> EPAENSDFYLPGDYLLGGLFSLHANMKGIVHLNFLQVPMCKEYEVKVIGYNLMQAMRFAVEEINNDSSLLPGVLLGYEIVDVCYISNNVQPVLYFLAHEDNLLPIQEDYSNYSSRVVAVIGPDNSESVMTVANFLSLFLLPQITYSAISDELRDKVRFPALLRTTPSADHHIEAMVQLMLHFRWNWIIVLVSNDTYGRDNGQLLGERVARRDICIAFQETLPTLQPNQNMTSEERQRLVTIVDKLQQSTARVVVVFSPDLTLYHFFNEVLRQNFTGAVWIASESWAIDPVLHNLTELRHLGTFLGITIQSVPIPGFSEFREWGPQAGPPPLSRTSQSYTCNQECDNCLNATLSFNTILRLSGERVVYSVYSAVYAVAHALHSLLGCDKSTCTKRVVYPWQLLEEIWKVNFTLLDHQIFFDPQGDVALHLEIVQWQWDRSQNPFQSVASYYPLQRQLKNIQDISWHTINNTIPMSMCSKRCQSGQKKKPVGIHVCCFECIDCLPGTFLNHTEDEYECQACPNNEWSYQSETSCFKRQLVFLEWHEAPTIAVALLAALGFLSTLAILVIFWRHFQTPIVRSAGGPMCFLMLTLLLVAYMVVPVYVGPPKVSTCLCRQALFPLCFTICISCIAVRSFQIVCAFKMASRFPRAYSYWVRYQGPYVSMAFITVLKMVIVVIGMLATGLSPTTRTDPDDPKITIVSCNPNYRNSLLFNTSLDLLLSVVGFSFAYMGKELPTNYNEAKFITLSMTFYFTSSVSLCTFMSAYSGVLVTIVDLLVTVLNLLAISLGYFGPKCYMILFYPERNTPAYFNSMIQGYTMRRD;> LCLSQQFKAQGDYILGGLFPLGSTEEATLNQRTQPNSIPCNRFSPLGLFLAMAMKMAVEEINNGSALLPGLRLGYDLFDTCSEPVVTMKSSLMFLAKVGSQSIAAYCNYTQYQPRVLAVIGPHSSELALITGKFFSFFLMPQVSYSASMDRLSDRETFPSFFRTVPSDRVQLQAVVTLLQNFSWNWVAALGSDDDYGREGLSIFSSLANARGICIAHEGLVPQHDTSGQQLGKVLDVLRQVNQSKVQVVVLFASARAVYSLFSYSIHHGLSPKVWVASESWLTSDLVMTLPNIARVGTVLGFLQRGALLPEFSHYVETHLALAADPAFCASLNAELDLEEHVMGQRCPRCDDIMLQNLSSGLLQNLSAGQLHHQIFATYAAVYSVAQALHNTLQCNVSHCHVSEHVLPWQLLENMYNMSFHARDLTLQFDAEGNVDMEYDLKMWVWQSPTPVLHTVGTFNGTLQLQQSKMYWPGNQVPVSQCSRQCKDGQVRRVKGFHSCCYDCVDCKAGSYRKHPDDFTCTPCNQDQWSPEKSTACLPRRPKFLAWGEPVVLSLLLLLCLVLGLALAALGLSVHHWDSPLVQASGGSQFCFGLICLGLFCLSVLLFPGRPSSASCLAQQPMAHLPLTGCLSTLFLQAAETFVESELPLSWANWLCSYLRGLWAWLVVLLATFVEAALCAWYLIAFPPEVVTDWSVLPTEVLEHCHVRSWVSLGLVHITNAMLAFLCFLGTFLVQSQPGRYNRARGLTFAMLAYFITWVSFVPLLANVQVAYQPAVQMGAILVCALGILVTFHLPKCYVLLWLPKLNTQEFFL

Sugars and other sweet-tasting compounds are detected by the sweet taste receptor, a member of the class C GPCR family. The sweet receptor is a heterodimer composed of TAS1R2 and TAS1R3,3,4 two type 1 taste receptor family members that share the distinctive architecture of class C GPCRs: a large extracellular Venus flytrap (VFT) domain, responsible for ligand recognition; a cysteine-rich domain (CRD); and a seven-transmembrane (7TM) domain that mediates G protein coupling. To address this gap, here we present cryo-electron microscopy (cryo-EM) structures of the sweet receptor in the inactive, unliganded state, as well as in the activated, sucralose- and advantame-bound states. Unlike other class C GPCRs, such as mGluR, CaSR and GABAB receptors, where agonists stabilize inter-subunit VFT interactions to promote activation, the sweet receptor is activated by the rearrangement of a TAS1R2 VFT loop, which destabilizes interactions between the lower VFT lobes and the VFT–CRD interfaces.

We first determined the structure of the human/mouse sweet receptor in the absence of sweeteners. Through 3D classification, we observed substantial intrinsic mobility of the receptor. The extracellular domains tilt toward or away from the membrane, with an angular range of up to 11°. While the orientation between extracellular and transmembrane domains can vary, each domain remains nearly identical across individual classes. To improve the resolution, we combined all particles to generate a global reconstruction at 3.1 Å resolution, then performed local refinement focused on the VFT/CRD region or the 7TM domain, obtaining final resolutions of 2.9 Å and 3.6 Å, respectively. In the unliganded (apo) state, TAS1R2 and TAS1R3 show a highly asymmetric architecture, and their extracellular domains are markedly tilted relative to the membrane plane. These features differ from other heteromeric class C GPCRs, such as GABAB receptor and heteromeric mGluRs, which adopt an orientation perpendicular to the membrane plane. In our apo sweet receptor structure, the two subunits pack closely against each other at both the upper and lower lobes of the VFT domains, as well as at the 7TM domains. The tight packing of the sweet receptor is facilitated by interactions between VFT domains and CRDs, with the VFT LB2s held together by loops extending from the CRDs.>MHHHHHHMIKKEKRPPQTLSRGWGDDITWVQTYEEGLFYAQKSKKPLMVIHHLEDCQYSQALKKVFAQNEEIQEMAQNKFIMLNLMHETTDKNLSPDGQYVPRIMF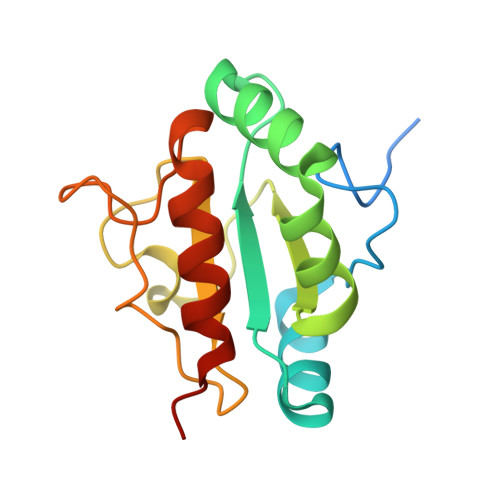VDPSLTVRADIAGRYSNRLYTYEPRDLPLLIENMKKALRLIQSEL[2x]SAP05 binds both the von Willibrand factor type A (vWA) domain of Rpn10 and the zinc-finger (ZnF) domain of multiple members of two distinct plant transcription factor families, known as SQUAMOSA-PROMOTER BINDING PROTEIN-LIKE (SPL) and GATA BINDING FACTORS (GATAs). The SAP05 protein comprises a globular compact structure with five β-strands that form an internal triangular mixed β-sheet core. β-strand 1 (β1) locates on the long end of this triangular core and connects via a loop–helix–loop–helix–loop structure to β2 at the opposite surface near the tip of this core. The SAP05 residues binding ZnF and vWA are located at opposing surfaces of the effector with the ZnF binding surface comprising the loop-dominated surface (loop surface) and the vWA-binding surface the β-sheet-dominated long end of the triangular β-sheet core (sheet surface). Our data show how the bacterial SAP05 effector has evolved as a functional adapter of the 26S proteasome to bypass the canonical UPS cellular proteolysis pathway and enable ubiquitin-independent degradation of structured eukaryotic proteins.

As Rpn10vWA formed aggregates upon purification in the absence of SAP05, Rpn10vWA was coexpressed with SAP05 and purified as a complex using the same general method. The SAP05 sheet surface comprises two parallel β-strands, β1 and β5, as well as two loops separated by an α-helix. The interaction is mediated by eight SAP05 amino acids, including R43 and N48 located on β1, S50 on loop 2, H58 on loop 3, T60 on α2, N125 and Y127 on β5, and Y132 on the loop following β5 of SAP05. Each of these residues interacts with one residue of Rpn10vWA, except for T60 that interacts with two residues, and S50 and H58 form two interactions with E31 and N34 of Rpn10vWA, respectively. Four of the interactions involve double or single hydrogen bonds and one salt bridge, and other interactions comprise nonbonded contacts. All Rpn10vWA residues that interact with SAP05 locate on α-helices. The Rpn10vWA interaction is largely mediated by polar forces. Thus, the SAP05 sheet surface contains rigid secondary β-sheets and α-helix structures that are held in place by hydrogen bonds within SAP05, as opposed to the ZnF-binding loop surface that involves protruding loop structures that may be more flexible. Structural superimposition of SAP05 interactions with vWA domains of plant Rpn10 and PSMD4 revealed that SAP05 loop 3 clashes with H38 of PSMD4 precluding a SAP05-PSMD4 interaction. The structural superposition of SAP05–Rpn10vWA complex onto the spinach 26S proteasome did not reveal obvious steric clashes with proteasome components.

> GPAPNEEFVGDMRIVNVNLSNIDILKKHETFKKYFDFTLTGPRYNGNIAEFAMIWKIKNPPLNLLGVFFDDGTRDDEDDKYILEELKQIGNGAKNMYIFWQYEQK;> GPVLEATMICIDNSEWMRNGDYSPSRLQAQTEAVNLLCGAKTQSNPENTVGILTMAGKGVRVLTTPTSDLGKILACMHGLDVGGEINLTAAIQIAQLALKHRQNKNQRQRIIVFAGSPIKYEKKALEIVGKRLKKNSVSLDIVNFGEDDDEEKPQKLEALLTAVNNNDGSHIVHVPSGANALSDVLLSTPVFTG>GHMAKHQIGVIGLAVMGKNLALNIESKGYSVAVYNRLREKTDEFLQEAKGKNIVGTYSIEEFVNALEKPRKILLMVKAGAPTDATIEQLKPHLEKGDIVIDGGNTYFKDTQRRNKELAELGIHFIGTGVSGGEEGALKGPSIMPGGQKEAHELVRPIFEAIAAKVDGEPCTTYIGPDGAGHYVKMVHNGIEYGDMQLIAEAYFLLKHVLGMDAAELHEVFADWNKGELNSYLIEITADIFTKIDEETGKPLVDVILDKAGQKGTGKWTSQNALDLGVPLPIITESVFARFLSAMKDERVKASKVLAGPAVKPFEGDRAHFIEAVRRALYMSKICSYAQGFAQMKAASEEYNWNLRYGDIAMIFRGGCIIRAQFLQKIKEAYDRDPALSNLLLDSYFKDIVERYQDALREIVATAAMRGIPVPGSA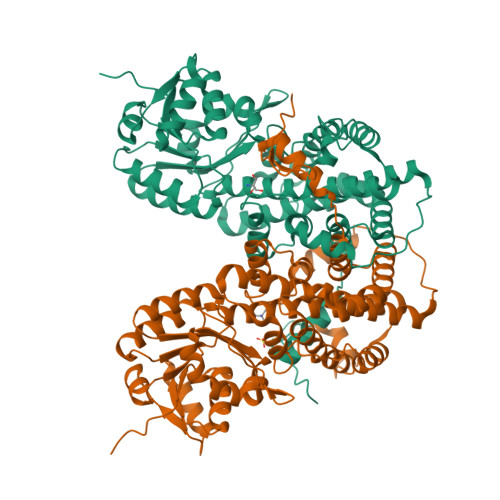SALAYYDSYRTAVLPANLIQAQRDYFGAHTYERVDKEGIFHTEWLK[2x]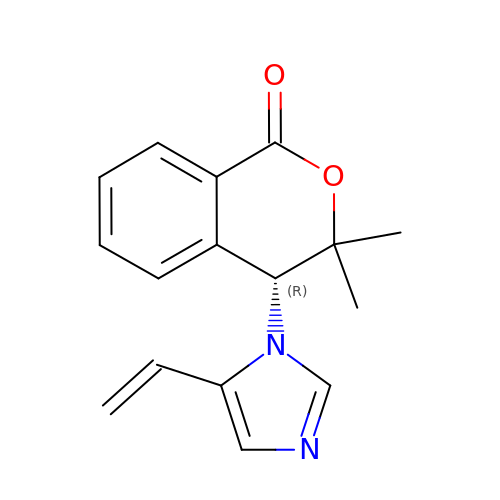(4R)-4-(5-ethenyl-1H-imidazol-1-yl)-3,3-dimethyl-3,4-dihydro-1H-2-benzopyran-1-one | C16 H16 N2 O2 | OENGIJBYVFYSCZ-CQSZACIVSA-N> GSRFVVEKNNLKVTSPDSIKGIYECAIGNFGVPQYGGTLVGTVVYPKSNQKACKSYSDFDISFKS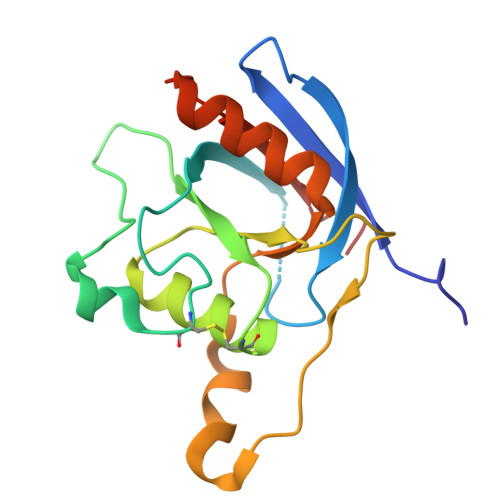KPGRLPTFVLIDRGDCYFTLKAWIAQQAGAAAILVADSKAEPLITMDTPEEDKSDADYLQNITIPSALITKTLGDSIKSALSGGDMVNMKLDWTESVPHP>[2x]GEFNTIQQLMMILNSASDQPSENLISYFNNCTVNPKESILKRVKDIGYIFKEKFAKAVGQGCVEIGSQRYKLGVRLYYRVMESMLKSEEERLSIQNFSKLLNDNIFHMSLLACALEVVMATYSRSTSQNLDSGTDLSFPWILNVLNLKAFDFYKVIESFIKAEGNLTREMIKHLERCEHRIMESLAWLSDSPLFDLIKQSKDREGPTDHLESACPLNLPLQNNHTAADMYLEPVRAPKKKSTSLSLFYKKVYRLAYLRLNTLCERLLSEHPELEHIIWTLFQHTLQNEYELMRDRHLDQIMMCSMYGICKVKNIDLKFKIIVTAYKDLPHAVQETFKRVLIKEEEYDYIIVFYNSVFMQRLKTNILQYASTRPPTLAPIPHIPRSPYKFP

The retinoblastoma tumor suppressor (Rb) is a multifunctional protein that primarily regulates the cell cycle but also has roles in cellular differentiation, DNA damage response, and apoptosis. Essential functions of Rb occur through its pocket domain, which is necessary for regulating binding interactions with E2F transcription factors and transcription repressors that bind via an LxCxE motif. The pocket domain is the most highly conserved region of the multidomain protein, as well as the most frequent site of mutations. Protein X-ray crystallography of four missense variants reveals how mutations destabilize the protein fold and inhibit E2FTD or LxCxE binding.

For a structural example of E7LxCxE inhibition, S751Y was crystallized. This variant weakens both E2F1TD and E7LxCxE binding relative to WT but causes the greatest reduction to E7LxCxE binding of all 75 missense variants tested here. The biggest reduction in E7LxCxE binding occurs for S751Y, which weakens the RbP–E7LxCxE binding interaction relative to WT by approximately 26-fold at 25 °C and 35-fold at 37 °C. The structure of S751Y reveals that the tyrosine sidechain of the mutant sits within a hydrophobic-binding pocket used for LxCxE binding. Specifically, the tyrosine sits in a position to compete for the binding of a conserved I or L, which constitutes a significant part of the LxCxEx(I/L)-binding epitope. Even though the variant tyrosine creates a snug fit into the pocket used for I/L binding, this variant is not stabilizing; instead, it causes a large destabilizing effect (ΔTm = −5.4 ± 0.5 °C). In the structure of WT Rb-E7LxCxE, the S751 sidechain helps to stabilize the N-terminus of an alpha helix through an ST motif–stabilizing H-bond to the amide at i+3. Loss of this known helix-stabilizing motif may be responsible for the large thermostability decrease seen for S751Y.Rhizobium etli, a nitrogen-fixing bacterial symbiont of legume plants, encodes an essential l-asparaginase (ReAV) with no sequence homology to known enzymes with this activity. High-resolution crystal structures of ReAV show indeed a structurally distinct, dimeric enzyme, with some resemblance to glutaminases and β-lactamases. The active site of ReAV, deduced from structural comparisons and confirmed by mutagenesis experiments, contains a highly specific Zn2+ binding site without a catalytic role. There are two Ser-Lys tandems, all connected through a network of H-bonds to the Zn center, and three tightly bound water molecules near Ser48, which clearly indicate the catalytic nucleophile.

The orthorhombic (OP) and monoclinic MP1/MP2 forms show similar packing pattern with solvent content of 49.4–52.6%, whereas the monoclinic form MC, with a significantly different arrangement of the dimers in the unit cell, has 53.2% solvent content. In the close vicinity of the Ser48 hydroxyl, there is a characteristic, almost tetrahedral pattern of three closely-spaced water molecules w2, w3, w4, visible in all crystal structures, except MP2. These waters must have extremely strong H-bonds with the Oγ atom of Ser48, as indicated by the O···O distances, which in the highest-resolution structure OP refined to 2.2–2.5 Å. The water molecules are also tightly H-bonded to each other. Water w3 is also H-bonded to w1 coordinated by the Zn2+ cation. The attraction of the three water molecules w2-w3-w4 by the Ser48 side chain is a clear evidence of this polarization. In the absence of a substrate, the arrangement of w2-w3-w4 might mimic the tetrahedral transition state of the catalytic event.

>[2x]GIDPFTMTPSEDFVVTDRGGIVENSHRVHAAVVDAKGRLLYALGNPTRMTLARSAAKPAQALAILETEGVAGYGFDDADIALMCASHSSEDRHIARTRAMLSKIKAEEADLRCGGHPSLSEMVNRSWIKQDFIPTAVCSNCSGKHVGMLAGARAIGAGTDGYHLPDHPMQGRVKRTVAELCDLDAGDVEWGTDGCNLPTPAFPLDRLGRIYAKLASAADGSDAGEGQSTRCAALAHIFRAMARHPEMVAGEGRYCTMLMRAFDGALVGKLGADASYAIGVRASDATRQLGTDGALGISVKIEDGNLEMLYAVVTELLERLGIGSPDVRSQLASFHHPQRVNTMGVTTGGVSFPFKLRGSKSNVDDPRLAAVAR>[4x]MNYQNDDLRIKEIKELLPPVALLEKFPATENAANTVAHARKAIHKILKGNDDRLLVVIGPCSIHDPVAAKEYATRLLALREELKDELEIVMRVYFEKPRTTVGWKGLINDPHMDNSFQINDGLRIARKLLLDINDSGLPAAGEFLD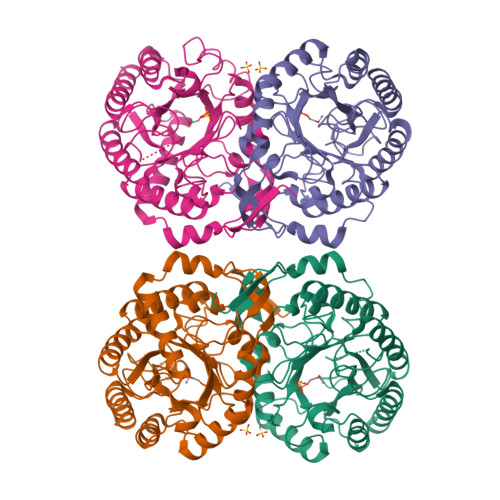MITPQYLADLMSWGAIGARTTESQVHRELASGLSCPVGFKNGTDGTIKVAIDAINAAGAPHCFLSVTKWGHSAIVNTSGNGDCHIILRGGKEPNYSAKHVAEVKEGLNKAGLPAQVMIDFSHANSSKQFKKQMDVCADVCQQIAGGEKAIIGVMVESHLVEGNQSLESGEPLAYGKSITDACIGWEDTDALLRQLANAVKARRG> ELYGASPDIDLGTGPTPTLGPVTPEICKQDIVFDGIAQIRGEIFFF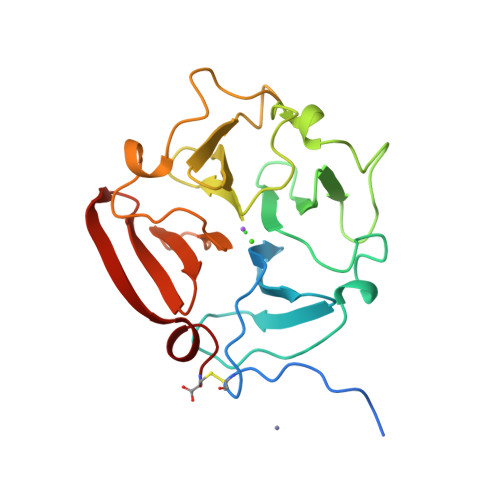KDRFIWRTVTPRDKPMGPLLVATFWPELPEKIDAVYEAPQEEKAVFFAGNEYWIYSASTLERGYPKPLTSLGLPPDVQRVDAAFNWSKNKKTYIFAGDKFWRYNEVKKKMDPGFPKLIADAWNAIPDNLDAVVDLQGGGHSYFFKGAYYLKLENQSLKSVKFGSIKSDWLGC>[2x]MAYTLPQLPYAYDALEPNIDAQTMEIHHTKHHQTYINNVNAALEGTEYADLPIEELVSKLKSLPENLQGPVRNNGGGHANHSLFWTVLSPN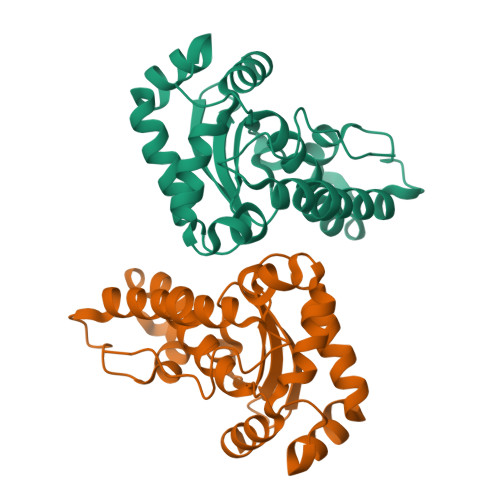GGGEPKGEVAKAIDKDLGGFEKFKEAFTKAAVSRFGSGWAWLSVTPDKKLVVESTANQDSPLFEGNTPILGLDVWEHAYYLKYQNRRPEYIGAFYNAVNWEEVERRYHAAIA>MNGKIALEEHFATEETLMDSAGFVPDKDWPELRSRLLDIQDRRVRLMDEHGIETMILSLNAPAVQAIADSTRANETARRANDFLAEQVAKQ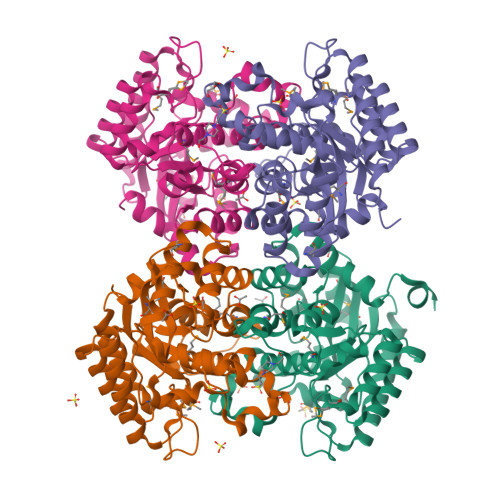PTRFRGFAALPMQDPELAARELERCVKELGFVGALVNGFSQDNRSAVPLYYDMAQYWPFWETVQALDVPFYLHPRNPLPSDARIYDGHAWLLGPTWAFGQETAVHALRLMGSGLFDKYPALKIILGHMGEGLPYSMWRIDHRNAWIKTTPKYPAKRKIVDYFNENFYLTTSGNFRTQTLIDAILEIGADRILFSTDWPFENIDHAADWFENTSISEADRKKIGWGNAQNLFKLNRAENLYFQSHHHHHHWSHPQFEK[8x]>[7x]MANFTPSRLGLVNNTGTGVKDLFLKTFAG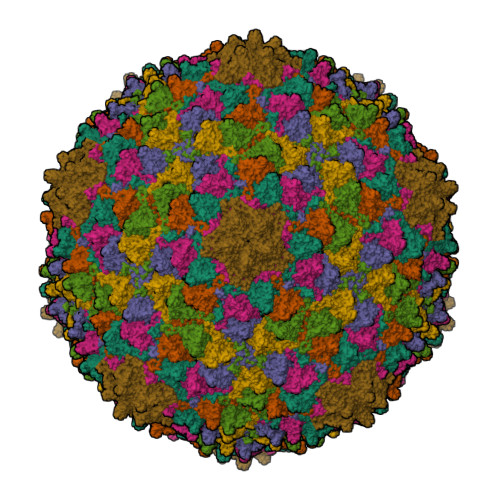EVLSAFRKATIFEDLHTVRTISSGKSAQFPIVGLSSTSYHSPGTQLTGNAIKHAEAVINIDDKLVSNVFIADVDEAMNHYDVRSQYSVQMGNALAYTFDQNVAAMIAQAARTSTNPNTDLPGGTRIKILKSGTANTAAAVAAVTGTDLATALFSAAEQMDINNLPEEDRYCAIDPTNYYKLVQNTTVINRDFGGRGAYAEGEVLKVAGIHIVKSNHLPKTNRSAATGENNTYHANYTDNIGLVFNKQAVGTVKLMDLKMEQTGADIHALYQGTFMVGSMMHGSGVLRPDCAIELYAANS> GPLGSTEVLCLMNMVLPEELLDDEEYEEIVEDVRDECSKYGLVKSIEIPRPVDGVEVPGCGKIFVEFTSVFDCQKAMQGLTGRKFANRVVVTK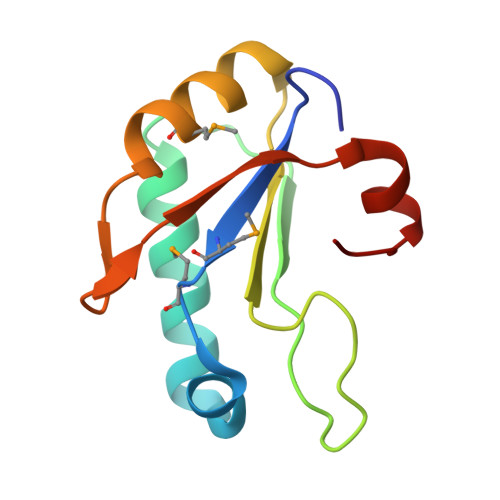YCDPDSYHRRDFW>[2x]MTTVYYDQDVKTDALQGKKIAVVGYGSQGHAHAQNLKDNGYDVVIGIRPGRSFDKAKEDGFDVFPVAEAVKQADVIMVLLPDEIQGDVYKNEIEPNLEKHNALAFAHGFNIHFGVIQPPADVDVFLVAPKGPGHLVRRTFVEGSAVPSLFGIQQDASGQARNIALSYAKGIGATRAGVIETTFKEETETDLFGEQAVLCGGVSKLIQSGFET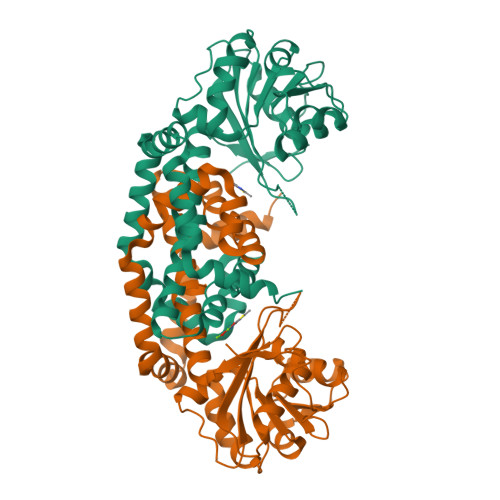LVEAGYQPELAYFEVLHEMKLIVDLMYEGGMENVRYSISNTAEFGDYVSGPRVITPDVKENMKAVLTDIQNGNFSNRFIEDNKNGFKEFYKLREEQHGHQIEKVGRELREMMPFIKSKSIEKHHHHHH In malignancies with wild type p53 status, the activity of p53 is commonly attenuated through overexpression of Mdm2, a key negative regulator. Mdm2 both inhibits the transactivation function of p53 and selectively ubiquitinates p53, targeting it for proteosomal degradation. Binding is achieved by recapitulating interactions of three key p53 amino acid side chains (F19, W23, L26), with discrete pockets lining the hydrophobic cleft. We have previously described the mutations M62A and Q24R in the N-terminal domain of Mdm2 that impart Nutlin-resistance by selectively reducing affinity for Nutlin but not p53. Here, we present the three dimensional crystal structure of a stapled peptide antagonist bound to Nutlin-resistant mutant Mdm2.

The structure of M06 in complex with Mdm2-M62A was elucidated using X-ray crystallography, revealing 2 complexes in the asymmetric unit of the crystal. The p53 peptide binding groove in both complexes was occupied by a single molecule of M06, where electron density in the 2Fo-Fc could be observed for the entirety of both molecules. Additionally, in the Mdm2-M62A:M06 crystal structure the peptide binding groove is capped by the helical ‘hinge’ region of the lid (residues 20–24), where the C-terminus of the stapled peptide packs. This helical region of Mdm2 interacts with the C-terminal amide group of M06 by forming hydrogen bonds via Q24. Interestingly, the greater helicity observed in the C-terminal helical turn of the stapled peptide results in significant alteration of the C-alpha position of L26. The L26 side chain packs into the peptide groove in an orientation that is very different from its conformations in the p53 WT and PMI unstapled peptides. Apart from attenuating the binding of Nutlin, the M62A mutation also causes a significant change in the conformation of the aliphatic staple. The absence of the methionine side chain in Mdm2-M62A causes the conformation of the staple to change as it packs more closely against G58. The plasticity of the stapled peptide enables it to respond to the M62A mutation by making compensatory contacts. The capping of the binding pocket by the Mdm2 ‘hinge’ helix is stabilized via hydrogen bond interactions between Q24 and the C-terminal amide of M06. It is clear that this movement of the ‘hinge’ can be accommodated by the Y100 either projecting into (‘closed’ conformation) or out (‘open’ conformation) of the Mdm2 binding pocket.

>[2x]MSVPTDGAVTTSQIPASEQETLVRPKPLLLKLLKSVGAQKDTYTMKEVLFYLGQYIATKRLYDEKQQHIVYCSNDLLGDLFGVPSFSVKEHRKIYTMIYRNLVVVNQQESSDSGTSVSEN> TAPKSRNLFERNPNKELKPGENSPRQTPIFDPTVHWLFTTCGASGPHGPTQAQCNNAYQNSNLSVEVGSEGPLKGIQIWKVPATDTYSISGYGAAGGKGGKNTMMRSHGVSVLGIFNLEKDDMLYILVGQQGEDACPSTNQLIQKVCIGENNVIEEEIRVNRSVHEWAGGGGGGGGATYVFKMKDGVPVPLIIAAGGGGRAYGAKTDTFHPERLENNSSVLGLNGNSGAAGGGGGWNDNTSLLWAGKSLQEGATGGHSCPQAMKKWGWETRGGFGGGGGGCSSGGGGGGYIGGNAASNNDPEMDGEDGVSFISPLGILYTPAL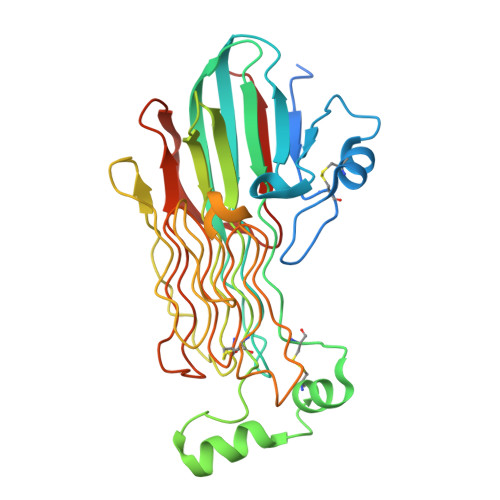KVMEGHGEVNIKHYLGTDEVD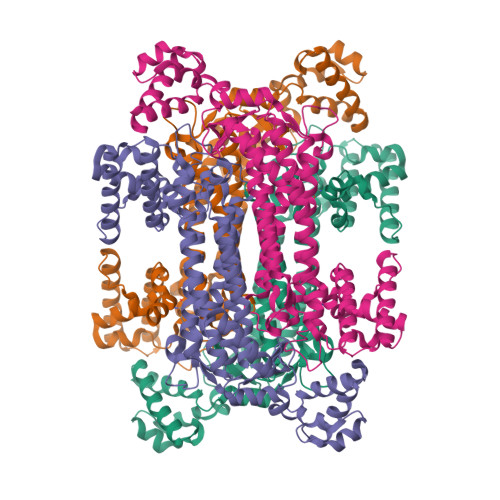>[4x]MAHRTWGGRFGEGPDALAARFNASLAFDRALWREDLWQNRVHARMLHAVGLLSAEELEAILKGLDRIEEEIEAGTFPWREELEDVHMNLEARLTELVGPPGGKLHTARSRNDQVATDLRLYLRGAIDELLALLLALRRVLVREAEKHLDPLYVLPGYTHLQRAQPVLLAHWFLAYYEMLKRDAGRLEDAKERLNESPLGAAALAGTGFPIDRHFTARELGFKAPMRNSLDAVASRDFALEVLSALNIGMLHLSRMAEELILYSTEEFGFVEVPDAFATGSSIMPQKKNPDILELIRAKAGRVLGAFVGLSAVVKGLPLAYNKDLQEDKEPLLDALATYRDSLRLLAALLPGLKWRRERMWRAAEGGYTLATELADYLAEKGLPFREAHHVVGRLVRRLVEEGRALKDLTLEELQAHHPLFAEDALPLLRLETAIHRRRSYGGTAPEAVRERLEEAKKEVGLD> SMKLDIKKTFSNRSDRVKGIDFHPTEPWVLTTLYSGRVEIWNYETQVEVRSIQVTETPVRAGKFIARKNWIIVGSDDFRIRVFNYNTGEKVVDFEAHPDYIRSIAVHPTKPYVLSGSDDLTVKLWNWENNWALEQTFEGHEHFVMCVAFNPKDPSTFASGCLDRTVKVWSLGQSTPNFTLTTGQERGVNYVDYYPLPDKPYMITASDDLTIKIWDYQTKSCVATLEGHMS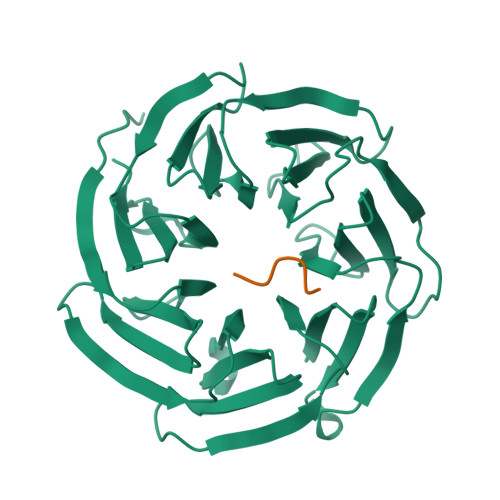NVSFAVFHPTLPIIISGSEDGTLKIWNSSTYKVEKTLNVGLERSWCIATHPTGRKNYIASGFDNGFTVLSLG;> GVKLHYT CCs are quaternary structures comprising two or more α-helices supercoiled around each other with cyclic (Cn) or dihedral (Dn) symmetry. Here, we describe variants with all combinations of the aliphatic residues, Ile, Leu and Val, at a and d to give four classes of peptide: the ββ class, with a and d = Ile or Val; Lβ, a = Leu and d = Ile or Val; βL, a = Ile or Val and d = Leu; and LL, a = d = Leu. Peptides are named systematically appending the one-letter code for the amino acids at the a and d sites to “CC-Type2-“; e.g., CC-Hept becomes CC-Type2-LI. In summary, solution-phase data and X-ray crystal structures demonstrate conclusively that different classes of Type-2 coiled-coil (CC) peptides—i.e., based on abcdefg repeats with predominantly hydrophobic residues at a, d, e and g—adopt a range of distinct states.

The combination of a = Leu plus d = Ile consistently forms α-helical barrels. First, the Leu residues at a were replaced by 4,5-dehydroleucine to give CC-Type2-deLI. This unnatural amino acid is similarly hydrophobicity to Leu, but it has an sp2 hybridised Cγ. In solution, this peptide behaved as a folded, heptameric, α-helical barrel. Indeed, its X-ray crystal structure overlaid almost precisely with the parent peptide CC-Type2-LI.

>XGEIAQAXKEIAKAXKEIAWAXKEIAQAXKGX[7x]2-chloranyl-6~{H}-thieno[2,3-b]pyrrole-5-carboxylic 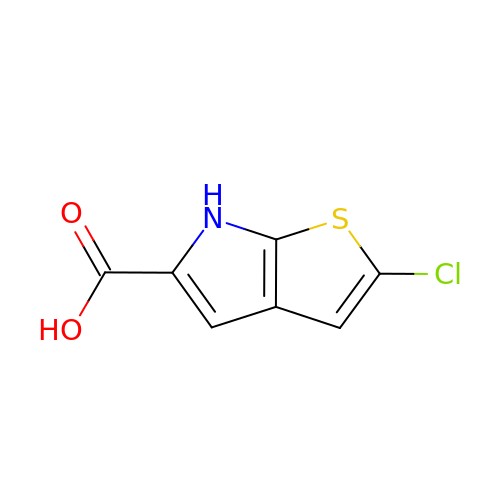acid | C7 H4 Cl N O2 S | SOGNHUJSAKAIRG-UHFFFAOYSA-N N-(1-CARBOXY-2-HYDROXY-4-OXO-BUTYL)-N-(3-OXO-CISPROPENYL)AMINE 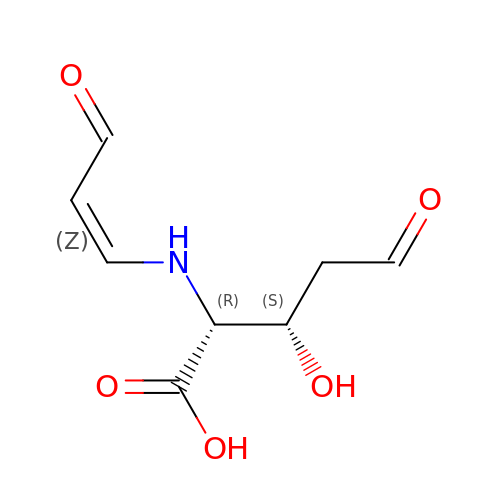| C8 H11 N O5 | DIQBZADGQQVQIO-WHFQOLMOSA-N2-methyl-5-(1-methylethyl)cyclohexa-2,5-diene-1,4-dione | 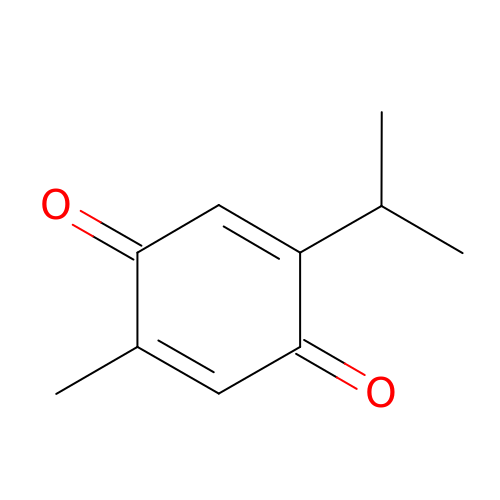C10 H12 O2 | KEQHJBNSCLWCAE-UHFFFAOYSA-N Cyanobacterial aldehyde-deformylating oxygenase (cADO), which catalyzes the conversion of Cn fatty aldehyde to its corresponding Cn-1 alk(a/e)ne, is a key enzyme in that pathway. Cyanobacterial aldehyde-deformylating oxygenase (cADO) belongs to the superfamily of ferritin-like di-iron proteins and contains a di-iron center. To gain insights into the reaction catalyzed by cADO, we determined structures of wild type ADO from Synechococcus elongates PCC7942 (Se) with different treatment (WT0, no treatment; WT1, co-crystallized with iron; WT-HP, soaked in H2O2), and solved the structures of two SeADO mutants (Y122F and F86YF87Y). SeADO belongs to the di-iron protein family, with conserved sequence of two EX28-29EX2H motifs, in which six conservative amino acids from four helices (Glu32 from helix H1, Glu115 from helix H4, Glu60 & His63 from helix H2, and Glu144 & His147 from helix H5) act as metal ligands.

Each asymmetric unit of WT0 crystal contains one SeADO molecule, and its active site appears to have lost both of its iron atoms. The WT0 structure is characterized by losing the di-iron cluster and by exhibiting a distorted conformation of helix H5. By contrast, the helix H5 is unwound in the middle in the structures of WT0 and molecule B of other three structures (WT1, F86YF87Y and WT-HP), forming two short helices (H5A and H5B) that are connected by a loop L5. The helix to loop transition results in a different conformation for a number of amino acids (from residue 144 to 150), thus the two iron-coordinating residues (Glu144 and His147) move away from the di-iron site. As a result, most of our SeADO structures with the L5 conformation lose their metal atoms. However, in the WT1 and WT0 structures, the electron density is consistent with a ligand with one single-head-group configuration, which is unlikely to be a fatty acid. We assume that if the loop conformation of helix H5, as revealed in the F86YF87Y structure, was not restored into a helical structure at the appropriate time, the solvent-accessible di-iron center may become unstable. Whereas the instability of the di-iron cluster further promotes the loop conformation, and thus results in a complete loss of the di-iron cluster, as shown in the WT0 structure. The structural flexibility of SeADO provides an explanation for its low iron occupancy, and may be in part responsible for the low enzymatic activity observed for cADO.

> MPQLEASLELDFQSESYKDAYSRINAIVIEGEQEAFDNYNRLAEMLPDQRDELHKLAKMEQRHMKGFMACGKNLSVTPDMGFAQKFFERLHENFKAAAAEGKVVTCLLIQSLIIECFAIAAYNIYIPVADAFARKITEGVVRDEYLHRNFGEEWLKANFDASKAELEEANRQNLPLVWLMLNEVADDARELGMERESLVEDFMIAYGEALENIGFTTREIMRMSAYGLAAV> AAAAGAAGCCACCCTCCCGTCACCGACTTGAG;> TCATAAATCAGTTCAGAAAACGAGTCTAGCTGTGCCTGAGTACAAAAT;> ATTCATTGAATCCCCAAGAATAACTTAATTAAATAAGGAGAAACCA;> CATTACCGAGGGGGTAATAGTACACTATCA;> AAAATCAGAAATCACCTCAAATCACCATCAATGTCTGGAGTTTTT;> TTTTTTAAATTTAAAGAAGATGATGATTTTTTAACAAACATCAAG;> AGCCAGCATGAGGGAGGATAAAAATTTTTAGATAATCGTACAAACAAG;> TTCTGACCAATATATTTTAATGGAAACAGTTTTTTTACATAAATCAAT;> CCAGAGCCGCCATCTTGGCATTTTCGGTCTTTTTTTTTTATAGCCCCCTTATCCATCGAT;> TTAGTTAAAAGACAAACCGCGCCCAATAGCATCGTAGG;> TGATAGACGGTTTTTCGCCCTTTGACGTTGGAGTCCACGTTCTTTAATAGTGGACTCTTGTTCCAAACTGGAACAACACTCAACCCTATCTCGGGCTATTCTTTTGATTTATAAGGGATTTTGCCGATTTCGGAACCACCATCAAACAGGATTTTCGCCTGCTGGGGCAAACCAGCGTGGACCGCTTGCTGCAACTCTCTCAGGGCCAGGCGGTGAAGGGCAATCAGCTGTTGCCCGTCTCACTGGTGAAAAGAAAAACCACCCTGGCGCCCAATACGCAAACCGCCTCTCCCCGCGCGTTGGCCGATTCATTAATGCAGCTGGCACGACAGGTTTCCCGACTGGAAAGCGGGCAGTGAGCGCAACGCAATTAATGTGAGTTAGCTCACTCATTAGGCACCCCAGGCTTTACACTTTATGCTTCCGGCTCGTATGTTGTGTGGAATTGTGAGCGGATAACAATTTCACACAGGAAACAGCTATGACCATGATTACGAATTCGAGCTCGGTACCCGGGGATCCTCAACTGTGAGGAGGCTCACGGACGCGAAGAACAGGCACGCGTGCTGGCAGAAACCCCCGGTATGACCGTGAAAACGGCCCGCCGCATTCTGGCCGCAGCACCACAGAGTGCACAGGCGCGCAGTGACACTGCGCTGGATCGTCTGATGCAGGGGGCACCGGCACCGCTGGCTGCAGGTAACCCGGCATCTGATGCCGTTAACGATTTGCTGAACACACCAGTGTAAGGGATGTTTATGACGAGCAAAGAAACCTTTACCCATTACCAGCCGCAGGGCAACAGTGACCCGGCTCATACCGCAACCGCGCCCGGCGGATTGAGTGCGAAAGCGCCTGCAATGACCCCGCTGATGCTGGACACCTCCAGCCGTAAGCTGGTTGCGTGGGATGGCACCACCGACGGTGCTGCCGTTGGCATTCTTGCGGTTGCTGCTGACCAGACCAGCACCACGCTGACGTTCTACAAGTCCGGCACGTTCCGTTATGAGGATGTGCTCTGGCCGGAGGCTGCCAGCGACGAGACGAAAAAACGGACCGCGTTTGCCGGAACGGCAATCAGCATCGTTTAACTTTACCCTTCATCACTAAAGGCCGCCTGTGCGGCTTTTTTTACGGGATTTTTTTATGTCGATGTACACAACCGCCCAACTGCTGGCGGCAAATGAGCAGAAATTTAAGTTTGATCCGCTGTTTCTGCGTCTCTTTTTCCGTGAGAGCTATCCCTTCACCACGGAGAAAGTCTATCTCTCACAAATTCCGGGACTGGTAAACATGGCGCTGTACGTTTCGCCGATTGTTTCCGGTGAGGTTATCCGTTCCCGTGGCGGCTCCACCTCTGAAAGCTTGGCACTGGCCGTCGTTTTACAACGTCGTGACTGGGAAAACCCTGGCGTTACCCAACTTAATCGCCTTGCAGCACATCCCCCTTTCGCCAGCTGGCGTAATAGCGAAGAGGCCCGCACCGATCGCCCTTCCCAACAGTTGCGCAGCCTGAATGGCGAATGGCGCTTTGCCTGGTTTCCGGCACCAGAAGCGGTGCCGGAAAGCTGGCTGGAGTGCGATCTTCCTGAGGCCGATACTGTCGTCGTCCCCTCAAACTGGCAGATGCACGGTTACGATGCGCCCATCTACACCAACGTGACCTATCCCATTACGGTCAATCCGCCGTTTGTTCCCACGGAGAATCCGACGGGTTGTTACTCGCTCACATTTAATGTTGATGAAAGCTGGCTACAGGAAGGCCAGACGCGAATTATTTTTGATGGCGTTCCTATTGGTTAAAAAATGAGCTGATTTAACAAAAATTTAATGCGAATTTTAACAAAATATTAACGTTTACAATTTAAATATTTGCTTATACAATCTTCCTGTTTTTGGGGCTTTTCTGATTATCAACCGGGGTACATATGATTGACATGCTAGTTTTACGATTACCGTTCATCGATTCTCTTGTTTGCTCCAGACTCTCAGGCAATGACCTGATAGCCTTTGTAGATCTCTCAAAAATAGCTACCCTCTCCGGCATTAATTTATCAGCTAGAACGGTTGAATATCATATTGATGGTGATTTGACTGTCTCCGGCCTTTCTCACCCTTTTGAATCTTTACCTACACATTACTCAGGCATTGCATTTAAAATATATGAGGGTTCTAAAAATTTTTATCCTTGCGTTGAAATAAAGGCTTCTCCCGCAAAAGTATTACAGGGTCATAATGTTTTTGGTACAACCGATTTAGCTTTATGCTCTGAGGCTTTATTGCTTAATTTTGCTAATTCTTTGCCTTGCCTGTATGATTTATTGGATGTTAATGCTACTACTATTAGTAGAATTGATGCCACCTTTTCAGCTCGCGCCCCAAATGAAAATATAGCTAAACAGGTTATTGACCATTTGCGAAATGTATCTAATGGTCAAACTAAATCTACTCGTTCGCAGAATTGGGAATCAACTGTTATATGGAATGAAACTTCCAGACACCGTACTTTAGTTGCATATTTAAAACATGTTGAGCTACAGCATTATATTCAGCAATTAAGCTCTAAGCCATCCGCAAAAATGACCTCTTATCAAAAGGAGCAATTAAAGGTACTCTCTAATCCTGACCTGTTGGAGTTTGCTTCCGGTCTGGTTCGCTTTGAAGCTCGAATTAAAACGCGATATTTGAAGTCTTTCGGGCTTCCTCTTAATCTTTTTGATGCAATCCGCTTTGCTTCTGACTATAATAGTCAGGGTAAAGACCTGATTTTTGATTTATGGTCATTCTCGTTTTCTGAACTGTTTAAAGCATTTGAGGGGGATTCAATGAATATTTATGACGATTCCGCAGTATTGGACGCTATCCAGTCTAAACATTTTACTATTACCCCCTCTGGCAAAACTTCTTTTGCAAAAGCCTCTCGCTATTTTGGTTTTTATCGTCGTCTGGTAAACGAGGGTTATGATAGTGTTGCTCTTACTATGCCTCGTAATTCCTTTTGGCGTTATGTATCTGCATTAGTTGAATGTGGTATTCCTAAATCTCAACTGATGAATCTTTCTACCTGTAATAATGTTGTTCCGTTAGTTCGTTTTATTAACGTAGATTTTTCTTCCCAACGTCCTGACTGGTATAATGAGCCAGTTCTTAAAATCGCATAAGGTAATTCACAATGATTAAAGTTGAAATTAAACCATCTCAAGCCCAATTTACTACTCGTTCTGGTGTTTCTCGTCAGGGCAAGCCTTATTCACTGAATGAGCAGCTTTGTTACGTTGATTTGGGTAATGAATATCCGGTTCTTGTCAAGATTACTCTTGATGAAGGTCAGCCAGCCTATGCGCCTGGTCTGTACACCGTTCATCTGTCCTCTTTCAAAGTTGGTCAGTTCGGTTCCCTTATGATTGACCGTCTGCGCCTCGTTCCGGCTAAGTAACATGGAGCAGGTCGCGGATTTCGACACAATTTATCAGGCGATGATACAAATCTCCGTTGTACTTTGTTTCGCGCTTGGTATAATCGCTGGGGGTCAAAGATGAGTGTTTTAGTGTATTCTTTTGCCTCTTTCGTTTTAGGTTGGTGCCTTCGTAGTGGCATTACGTATTTTACCCGTTTAATGGAAACTTCCTCATGAAAAAGTCTTTAGTCCTCAAAGCCTCTGTAGCCGTTGCTACCCTCGTTCCGATGCTGTCTTTCGCTGCTGAGGGTGACGATCCCGCAAAAGCGGCCTTTAACTCCCTGCAAGCCTCAGCGACCGAATATATCGGTTATGCGTGGGCGATGGTTGTTGTCATTGTCGGCGCAACTATCGGTATCAAGCTGTTTAAGAAATTCACCTCGAAAGCAAGCTGATAAACCGATACAATTAAAGGCTCCTTTTGGAGCCTTTTTTTTGGAGATTTTCAACGTGAAAAAATTATTATTCGCAATTCCTTTAGTTGTTCCTTTCTATTCTCACTCCGCTGAAACTGTTGAAAGTTGTTTAGCAAAATCCCATACAGAAAATTCATTTACTAACGTCTGGAAAGACGACAAAACTTTAGATCGTTACGCTAACTATGAGGGCTGTCTGTGGAATGCTACAGGCGTTGTAGTTTGTACTGGTGACGAAACTCAGTGTTACGGTACATGGGTTCCTATTGGGCTTGCTATCCCTGAAAATGAGGGTGGTGGCTCTGAGGGTGGCGGTTCTGAGGGTGGCGGTTCTGAGGGTGGCGGTACTAAACCTCCTGAGTACGGTGATACACCTATTCCGGGCTATACTTATATCAACCCTCTCGACGGCACTTATCCGCCTGGTACTGAGCAAAACCCCGCTAATCCTAATCCTTCTCTTGAGGAGTCTCAGCCTCTTAATACTTTCATGTTTCAGAATAATAGGTTCCGAAATAGGCAGGGGGCATTAACTGTTTATACGGGCACTGTTACTCAAGGCACTGACCCCGTTAAAACTTATTACCAGTACACTCCTGTATCATCAAAAGCCATGTATGACGCTTACTGGAACGGTAAATTCAGAGACTGCGCTTTCCATTCTGGCTTTAATGAGGATTTATTTGTTTGTGAATATCAAGGCCAATCGTCTGACCTGCCTCAACCTCCTGTCAATGCTGGCGGCGGCTCTGGTGGTGGTTCTGGTGGCGGCTCTGAGGGTGGTGGCTCTGAGGGTGGCGGTTCTGAGGGTGGCGGCTCTGAGGGAGGCGGTTCCGGTGGTGGCTCTGGTTCCGGTGATTTTGATTATGAAAAGATGGCAAACGCTAATAAGGGGGCTATGACCGAAAATGCCGATGAAAACGCGCTACAGTCTGACGCTAAAGGCAAACTTGATTCTGTCGCTACTGATTACGGTGCTGCTATCGATGGTTTCATTGGTGACGTTTCCGGCCTTGCTAATGGTAATGGTGCTACTGGTGATTTTGCTGGCTCTAATTCCCAAATGGCTCAAGTCGGTGACGGTGATAATTCACCTTTAATGAATAATTTCCGTCAATATTTACCTTCCCTCCCTCAATCGGTTGAATGTCGCCCTTTTGTCTTTGGCGCTGGTAAACCATATGAATTTTCTATTGATTGTGACAAAATAAACTTATTCCGTGGTGTCTTTGCGTTTCTTTTATATGTTGCCACCTTTATGTATGTATTTTCTACGTTTGCTAACATACTGCGTAATAAGGAGTCTTAATCATGCCAGTTCTTTTGGGTATTCCGTTATTATTGCGTTTCCTCGGTTTCCTTCTGGTAACTTTGTTCGGCTATCTGCTTACTTTTCTTAAAAAGGGCTTCGGTAAGATAGCTATTGCTATTTCATTGTTTCTTGCTCTTATTATTGGGCTTAACTCAATTCTTGTGGGTTATCTCTCTGATATTAGCGCTCAATTACCCTCTGACTTTGTTCAGGGTGTTCAGTTAATTCTCCCGTCTAATGCGCTTCCCTGTTTTTATGTTATTCTCTCTGTAAAGGCTGCTATTTTCATTTTTGACGTTAAACAAAAAATCGTTTCTTATTTGGATTGGGATAAATAATATGGCTGTTTATTTTGTAACTGGCAAATTAGGCTCTGGAAAGACGCTCGTTAGCGTTGGTAAGATTCAGGATAAAATTGTAGCTGGGTGCAAAATAGCAACTAATCTTGATTTAAGGCTTCAAAACCTCCCGCAAGTCGGGAGGTTCGCTAAAACGCCTCGCGTTCTTAGAATACCGGATAAGCCTTCTATATCTGATTTGCTTGCTATTGGGCGCGGTAATGATTCCTACGATGAAAATAAAAACGGCTTGCTTGTTCTCGATGAGTGCGGTACTTGGTTTAATACCCGTTCTTGGAATGATAAGGAAAGACAGCCGATTATTGATTGGTTTCTACATGCTCGTAAATTAGGATGGGATATTATTTTTCTTGTTCAGGACTTATCTATTGTTGATAAACAGGCGCGTTCTGCATTAGCTGAACATGTTGTTTATTGTCGTCGTCTGGACAGAATTACTTTACCTTTTGTCGGTACTTTATATTCTCTTATTACTGGCTCGAAAATGCCTCTGCCTAAATTACATGTTGGCGTTGTTAAATATGGCGATTCTCAATTAAGCCCTACTGTTGAGCGTTGGCTTTATACTGGTAAGAATTTGTATAACGCATATGATACTAAACAGGCTTTTTCTAGTAATTATGATTCCGGTGTTTATTCTTATTTAACGCCTTATTTATCACACGGTCGGTATTTCAAACCATTAAATTTAGGTCAGAAGATGAAATTAACTAAAATATATTTGAAAAAGTTTTCTCGCGTTCTTTGTCTTGCGATTGGATTTGCATCAGCATTTACATATAGTTATATAACCCAACCTAAGCCGGAGGTTAAAAAGGTAGTCTCTCAGACCTATGATTTTGATAAATTCACTATTGACTCTTCTCAGCGTCTTAATCTAAGCTATCGCTATGTTTTCAAGGATTCTAAGGGAAAATTAATTAATAGCGACGATTTACAGAAGCAAGGTTATTCACTCACATATATTGATTTATGTACTGTTTCCATTAAAAAAGGTAATTCAAATGAAATTGTTAAATGTAATTAATTTTGTTTTCTTGATGTTTGTTTCATCATCTTCTTTTGCTCAGGTAATTGAAATGAATAATTCGCCTCTGCGCGATTTTGTAACTTGGTATTCAAAGCAATCAGGCGAATCCGTTATTGTTTCTCCCGATGTAAAAGGTACTGTTACTGTATATTCATCTGACGTTAAACCTGAAAATCTACGCAATTTCTTTATTTCTGTTTTACGTGCAAATAATTTTGATATGGTAGGTTCTAACCCTTCCATTATTCAGAAGTATAATCCAAACAATCAGGATTATATTGATGAATTGCCATCATCTGATAATCAGGAATATGATGATAATTCCGCTCCTTCTGGTGGTTTCTTTGTTCCGCAAAATGATAATGTTACTCAAACTTTTAAAATTAATAACGTTCGGGCAAAGGATTTAATACGAGTTGTCGAATTGTTTGTAAAGTCTAATACTTCTAAATCCTCAAATGTATTATCTATTGACGGCTCTAATCTATTAGTTGTTAGTGCTCCTAAAGATATTTTAGATAACCTTCCTCAATTCCTTTCAACTGTTGATTTGCCAACTGACCAGATATTGATTGAGGGTTTGATATTTGAGGTTCAGCAAGGTGATGCTTTAGATTTTTCATTTGCTGCTGGCTCTCAGCGTGGCACTGTTGCAGGCGGTGTTAATACTGACCGCCTCACCTCTGTTTTATCTTCTGCTGGTGGTTCGTTCGGTATTTTTAATGGCGATGTTTTAGGGCTATCAGTTCGCGCATTAAAGACTAATAGCCATTCAAAAATATTGTCTGTGCCACGTATTCTTACGCTTTCAGGTCAGAAGGGTTCTATCTCTGTTGGCCAGAATGTCCCTTTTATTACTGGTCGTGTGACTGGTGAATCTGCCAATGTAAATAATCCATTTCAGACGATTGAGCGTCAAAATGTAGGTATTTCCATGAGCGTTTTTCCTGTTGCAATGGCTGGCGGTAATATTGTTCTGGATATTACCAGCAAGGCCGATAGTTTGAGTTCTTCTACTCAGGCAAGTGATGTTATTACTAATCAAAGAAGTATTGCTACAACGGTTAATTTGCGTGATGGACAGACTCTTTTACTCGGTGGCCTCACTGATTATAAAAACACTTCTCAGGATTCTGGCGTACCGTTCCTGTCTAAAATCCCTTTAATCGGCCTCCTGTTTAGCTCCCGCTCTGATTCTAACGAGGAAAGCACGTTATACGTGCTCGTCAAAGCAACCATAGTACGCGCCCTGTAGCGGCGCATTAAGCGCGGCGGGTGTGGTGGTTACGCGCAGCGTGACCGCTACACTTGCCAGCGCCCTAGCGCCCGCTCCTTTCGCTTTCTTCCCTTCCTTTCTCGCCACGTTCGCCGGCTTTCCCCGTCAAGCTCTAAATCGGGGGCTCCCTTTAGGGTTCCGATTTAGTGCTTTACGGCACCTCGACCCCAAAAAACTTGATTTGGGTGATGGTTCACGTAGTGGGCCATCGCCC;> AACGGAGATTTGTATTAGGAATACAAAAGGATCAGGACGATGCCACT;> TTTTTGCGCGAAACACTAAAACCAGCGATAAGAGGCAGAGGACTAAAGACTTT;> TTGAGATTTTGTGAATTATACCAGAACGTAACCAGCATCGGAACGAGG;> CTGACCTTCATCGCCTCCATGTTAATTACGAGCGTTTACCAGACGACG;> GTAATCTTGACAAGATTGAAAGACTCCAAAACTAAAGGATTTTCACGGCTGAGGC;> TTTTGTTTTGTCCAGACAGCCCTCATTTTTTTTTTTAGTTAGCGTAAC;> AGACGTTAGTAAATGAATTGTATTCTTAAAC;> CGGTTTATCAGCTTGTTGAAAATTTTTT;> GTTTCAGCAGCTTGATCATCGCCCACGCATAAGCATGATTAACAGTTA;> GGAGTGAGTTGCGGGATCGTCACCCCCGTATA;> GTGAATAAGGCTTTTTTTTTTTTGCCCTGACGAGAAAACCCATGTCAGGGAT;> TCATTCATGGTTTAATTTCAACTTTAATCAAATTTTCT;> AAAGCTGCTTCAACAGTATGGGATTTTGCTGATCTAAAGCTTGAGA;> ACCGGATAGGAACAAAAAAGGCTCCAAAAGGAGCCTTTCATCAAGA;> GGTCAATCGACCAACTGAGGCTTTTTGCAGGGTTCGGAACCTATTATT;> TACGTTAATAAAATTTTTTTTTTCGAACTAACGGAACCTCATTTTTTT;> TTGGGAAGGGCTCATTACCTTATGCGATTTACACCAGATTACAGGT;> CAAAATAGCAGATACATAACGCCCACATTCAACTAATCAACATTATTTTT;> AAAAGCCTACCAGTATAAAGCCATATCATTCTGCAGAACGCTGAGAC;> TTACTAGACGGAATCGCCAACATGCAGAAGCAAAGCGGAT;> TTTTTCGTTAAATATGGTTTGAAATATTTTTTCCGACCGTGTGAT;> ACGAAGGCGTACCGACTTTTGCCAATTAGCAAGGCCGGAACCGTAATC;> AAAACGAAATCCGCGCGCAGACAGGCGCATAGGCTGG;> AAATTCTTGTTTAGTATCATATGAAAGAATAAAATGTTTAGCCAGTA;> CCATTAAATAGTACCGGTGCCGTCTTACCAGCGCCAAAGA;> TTCATGAGAACGAGGACCTGCTGATAAATTGTGTCGATATACCAATACAGACC;> GGTATTAAACCAAGTCGTTATACCATTTTCGAGACTGGA;> TCGGCTGTCTTTCCTACGCTCAATAACAACG;> CAGTACAACAATAGGTAAGAACTAAAAATCAGAAAGATTCATCAG;> CGCCTGTATTCGTCACAGTATAGCCCGGATTTTTTTTTTATAGGTGTATCAC;> GCCGCTTAATAGAAATTCATTACCCAAATCCTTAGCCGGGAAGTTT;> AGTTAAAGTTCGGTCCTTTCGAGGTGAATT;> CCAGCTACAGCGTCTTTCCAGAGTAGACGGGGAACAAAG;> TTTTGCATTCCAGGTAATAAGTTTTTTTTTTTTTTAACGGGGTCAGTG;> AAGACTCCAATACATACATAAAGGTGGAAAGCATAAATCC;> GAGGAAACGCTAACGAATTTTATCCTGAATACCGCACT;> TATCCCAACAGATATAGAGTACCTTTAATTGCTGTACCAACATTAACAGAACCTAC;> TATTATTGCCAGTTACAAGATTAGTTGCTATTATTTTC;> AACAGTGCTCAGCAGCAACAACACCGATAGTTGCGCCGTCTTTCC;> GAAGGCTTATCCGGTCCTTAAATCAAAATAGAACCTCCGAGAGAAT;> ATTCTAAGAACGCTTTTTTGAGGCGTTTTAGCATATAACTTAACCTCC;> GCGGATAAAAAAGGTAACGGAAATTATTCATT;> TTAGGATTCAATAAACGTTTTAATGTCTTTACGATTCAAAAGGGTGAG;> AAGCAAATGCGCCTGTAAGAGGAAGCCCGAAAAAATGCAAAAACATTA;> CAGCTAACAAGAACGACAAGCAAGCCGTTTTTTTGCACATTAAGAGTTACCAGA;> TTATCAACAATAGATATCAATAAAATCATTCCATCCTATTTTGAAG;> AAGTCCTGAACAATTTTTTGAAAAATAATATCAGAACGCGATGCAAAT;> AGAACCGCCACCCTTTTTTTTTTTCAGAGCCACCACTAGCGTTTTTTT;> ATATAAAACCAACCTTAACCCTGCATAGTAAGAGCAACAAAGTAC;> ATAAGAGACTGTCCAGACGACGAAGCGGGGT;> CCATATTCAGTAGGGACACCGGAATCATAA;> CAGGAAGAACAATAATTTGAATTACCTTTT;> ATGAATATTAGATTTTGTTATTAATTTTATTTTTTTTTTAAAGTTTGAGTAA;> GTAAACGTAGGGTTATCCAATAAATCATAC;> CCAATAGGTGTTAAATTCGGCCTCACCGCTTCCAGCAACCGCAAGAATTGGGTAAA;> ACTTCTGACATCTGCCCCGTCGGAAAGGGAAGAAAGCGAAAGCGGTCA;> TGGATTATCATATCAAAATTATTTTTGTATA;> GATTGTTGAGTCAATAGTGAATGGCTTAGGGACCATTGTTAAGCC;> TTTTTAACGCCATAACGGCGGATTGACCGCGGGGAAA;> AACTGTTGGGAAGTTTTTTTTTTGGCGATCGGTGCGTCGTCTCGTCCGGCAA;> GGCCTCTTCGCTATTCTTTGAATGATAATCTGACCCTG;> CAACCGATAAGACACCATAAAGCCTCAGAGCATTGTTAAACATATGTA;> CGGAAGCAAACTCCAACAGGTCAGAAAGATT;> GATACAGGGGAGGTTGCCTCAGAGCCGCCTTTTTTTTTTACCAGAACCACCAACCGGAAC;> GAAAATTCCGTAGAATTATTACGCAGTATGGACAATGAACTACAAAAACAACT;> TTTGTCACAATCAATAACAAACAAGCAGTCTC;> ACGGAATATATAAAATACCCAAAAGAACTGCCGATATA;> GTCATTTTTCGAGCTTTTTGCGGGAGAAGCCTTTATTTCATTAAGCA;> TTTTTAGTGTACTAGTAAGCGTCATATTTTTTTTTTCATGGCTTTTGATTTGGCCTT;> TGGCAACAAGTTTATATGCCCCCGTACCAGGTAGCAACGGCTACA;> GCTTAGAGCTTAATTAGGAAACCGATAGCCAGAATTAATGAGCGC;> GCTGAATACAACTAAAAGTAGTAGTAACCTGTTCTGGCCTTCCTGTAG;> TGAATTTACCGTTCCTTAGCAAACAGACGACCTTGAGTTGATATA;> ATTAAGACTCTGTAAAAGCAAATATTTAAATTGGCAAAGCAGTTTGAG;> ATAGCGATAGCTTAGTAGCTCAAGATTAGA;> TCATTAAAGCCGCCACAAAAGGGCGACATTTTTGCTCATGCCTAT;> TAAAGCTATAATACTCAAAGCGAACCAGACTCCTCAAGTGAAAGT;> AATCGGTTCCTTTTGATAAGAGCTGAAACAAGAAGGACATCGAGA;> TCGTCGCTATTAATTCCAATCGCTTGGGTTAACAGCCA;> AATTTTCCCTTAGTTTTTTAATCCTTGAAAACAAACAGAATCATCAAT;> CCACCACAGGCAGGTCAAAATCCGTACTCAGGAGGTTCGGGTAAACGAAAGA;> CCCTCAGAAACCGCCTCCCTCAGAAGTTTGCCCATTTGG;> ACCTTGCTCAATTTCACGGATTCGCCTGATTG;> ACCACCGGACCGCCACCCTCAGAGGATATTC;> ACCCTCATAGGTAAACCTGACTATAAATCATAGCGTCCAATACTG;> TTTCATCTTCATAATAATGAAAGCGAGAGGCTTTTGCATAAAAACATACGTA;> TCAGACTGTAGCGCGTCAGAGCCAAAGGTGAATATGGTGAGAGGGT;> CTTTAGCGAGTAGCGACAGAATCAGAGACAGAGTAGCACGAATTAG;> AAAGGCCGACGCAAGGGAAGGTAAATATTGAAGTAATT;> TAATGTGTATATTTTGACTTCAAATATCGCAACATGTTGCAGAGG;> ACATTTAAATAAATTATCTACAAAGGCTATCATAAAACGATGGCGAAA;> AGCAGCAACGTCACCATTATCAAGAACCGCCACCCTCAGCAAGCC;> ATGATATTCAACCGTAATGACCATTATAGTTAATTTAG;> ATGCCGGAGAGGGTACTCAAATGTTTCATCGAGAATCG;> CCCTGAACCTTACCAACGCAATAATAACGGAAGAAACGCA;> TTTTTAAAGTCAGATCTTACCGAAGCTTTTTTTTTTCCTTTTTAAGAAA;> TAATATCAGAGAGATAAAGAGCAATCCAAATATAAATATGTAATGCTG;> GAAATAGCAATAGCTAGGGTAATCTGAACA;> GAAACAATTCTGCGAACGAGTAGAATGGTCAAGCTGAGAA;> CAATAATACCCACAAAACAGGGAAGCGCATCCTAATTT;> AGAAACGATTTTTTGAACATAAAGAATTGACCTTT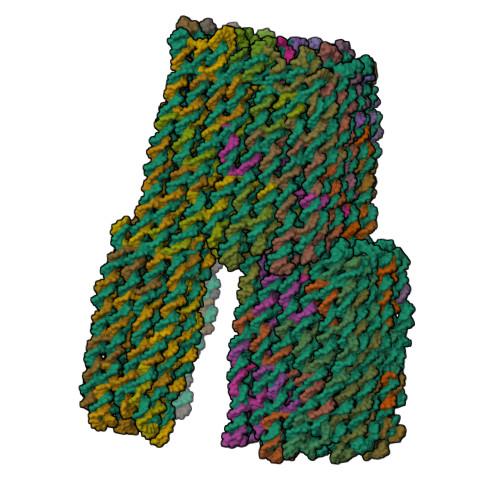ACATTTTT;> TTTAACGTCAAAATTTTTTATGAAAATAGCAGTACCTTTTTTTTT;> GTTTCATTTGCGGATGAGGCAAGGCAAAGAATTAGCAAAAGCCAGAA;> TTTTCCATATAATTTGGGGCGCGAGTTTTTTTTTTCTGAAAAGGTGGC;> TTAGCTATATTTTCACAGTTGATTCTGGAAAGTAAGCA;> AGATACATTTCGCAATTTAGTTTCATGTTT;> TTATCAAAATCATTTTTTTAGGTCTGAGAGACATGGCAATTTTTT;> TTTTTCTGAGCAAGAATTGAGGAAGGTTTTTTTTTTTTATCTAAAATAT;> CGCGCAGACAACTAATCGGCCAGTGAACGGATAACCTCAC;> ATTCATTAAAACAAAATTAATTTGCATCAACTTTAAA;> TCAATTACTTTTACATTACATTTGAGGATTTTTTTTTTTTTAGAAGTATTAG;> CGGGAGAAACGTCAGATATGTGAGTGAATA;> AGAAAAGCCCCAAAAACGACAACTAGATTAGATTTTGAAT;> CCTTCTGACTTGCTGGATTAGTAATAACATTTTTTTTTTTCACTTGCCTGAGTTTTTATA;> ACTTTCTCCGGCCTTTAGTGATGAAGGGTAAACTTAAATGAGACGCA;> AATTTGTGAGAGATAGCGGAAAAATTCTGCTC;> ATCGGCGCCAGTCACGACGTTGGGTCATTGACCAAGT;> TTTTTGTTGAAAGCTCAATCAATATCTTTTTTTTTTTGGTCAGTTGGCATACCGAAC;> TTTTTAAAAAAGCTTGGGCGGATAAAAAAAAGGGATAGCTCTCA;> ACTGATAGGGCTATTAATTCACCAGGAAAAACGCTCATGGCCATCAC;> CCCTAAAACAGCAGAATGCTGAACCTCAAATATCAAACCGTGGAGCC;> CATCGCCAGCCACGGGCCAAGCTTTCAGAGGCTATTTT;> TTAAAAACTTTAGGAGCACTAAGGCGAATTTGAGAGA;> ACGCCAGCGCCATTCGCACATCCTCATAACGG;> AGGCGATTGGGTTTTCAAACGTACAGCGCCAT;> GGGGGATGTGCTGCAAGAATCGACCTGAGA;> CAACAGCTCGTGCCAGCTGCTTTTTTTTTTATTAATGAATCGGCCAGTCGGTTCACGGT;> GGGAACACAAAAATATTTTTAAATCAATTCTACTAATGTACGGTGTCCCAAT;> GTAACAACAAACCACCTAAACAGGAGGCCGATGCCGCGCT;> GGGCGCCAGGATCCCCGGGTACCGCCTCCTC;> TAGATGGGGCCTGGGGTGCCTAATAAGCACTAGAGCTTGAGGGTCGAGTTTTT;> CGCATCGTAACCGTGATAATGGAATTCGCG;> ATCATCATATTCCTTTTTTTTTTTGATTATCAGATGGTGCTTTCTTTTT;> TCATGGTCATACCGGGGGTTTTTTTTTTTTTCTGCCAGCACGCGGGCCGTTTTTTT;> ATTCGTAACGGGGAGAGGCGGTTTCACCAGT;> AGGAAGATCAACATACGAGCCGGATCCCTTAC;> GAACAAAGCGTATTAATAGAACGTCAGCGTGGGCAAATTA;> ATCCTTTGCCCGAACCAGGTTTAGCACGTA;> CAGCTTAGTGCCTGTTCTTCGCGTCCGTGAGAGCTCGATGTGAAATGCGTTGCG;> GTCGGTGGTGCCATCCAGCATCAGCAGATGCCCCCTGCATTAAATCAA;> TGCTGGTCTTTTAGAGGGACGACGACAGTACAGCTCATTAATATT;> TGTTATCCAACGGCATCGGGGTCAGCGCGGTTCAGACGATCCAGCGCA;> GCTCACAACAGCACCACAGTTGAAGCCAGCTTTCCGGC;> AGCATAAATGGTCAGTGGTGCCGGAAACCA;> CAGGAACGGTACGCCAAGGCCACCACCGTTGT;> TAGAAGAACTCGTTAGACTATGGTCGTATAACGGCGCTGGCAAGTGT;> TTTTGAAACCTGTCCAGTTTGGAACTTTTTTTTTTAAGAGTCCACTAT;> GCCTGGCCCTGAGAGACCAGCAGGAAAGGGCGACGTGAACGCGGTATG;> AAGCGGTTAATGGGAGGGTGGTTTTTCTTTTGCGTATTCATTAATT;> GCCGGCGACCGATTTAAATCGGAACCCTAAAGATAAACA;> AGGAGCGGCGGGAGCAGAAGGAGCGGAATTATAATCCTCATCAAC;> TGGTGGTTGATTGCCCTTCACCGAGACGGG;> CGCTGCGCGTAACCACGGAGCCCACGTGGCGGTGTAAA;> GTGGACTCTCACTGCCCGCTTTCCAACGCG;> CCAACGTCCGAAAATCATCCCTTACATCACCCAAATCAAG;> TAATGCGCCGCTACAGATCAGTGGAATCCTGGGACTTG;> GGCGCGTAATCAGAGGCGCTAGATTAAATGTGAGCGACCAGCTTT;> CTGTGGTGCTGCGTTTTTTTTTTGCCAGAATGCGGCTGCGCGCCTTTT;> ACTGGTGTGCCCTGCGGTGCCGTAGGGCGATGGCCCACTAAAAACCGAATCGTT;> GAGTAAAAGAGTCTGTCACACCCTAAAGGGAAGAAAGGTTCTCCGT;> GCTTTCGGCCAACGGTTCCACACGCACTCCTAGGTCACGTTGGTG;> GGTTTCTTTGCTCGTCAAATACCAGCCTCCGCGTTTTT;> AGCAATACCCAGCCAAACGTGCCACAATATGCCGTCAATAGATAA;> TTCTTTGTAATATCCAGAAGTGCATTATCATTTTGCG;> GTGTCACCGGCTGGAGGTGTCCCACGCAACTTTCCTG;> TTTTTGCTGGTAACACTCAATCCGCCGGTTGCAGGC;> AGCCGGGTCACTGTTGTTCAGCATCTATCAGAGTGAGC;> TAGGGTTGTGTGCACTAGCGGTGCCGGTGCCGGGTTACC;> AAGAATAGCCCGAGATAAAGAACTGCAGCCCATAGCTG;> TTTTTAGTGTTGTTCCGAAATCGGCAAACTGTTTGA;> TTTTTTGCCACGCTGGTTTGCCGTTGCAGCTAACTCA;> TTGCAACAGTCACACGACCAGTAAGAACCAC;> TAAAAGGTGGCACAGAGAACAAACTTTACAAACAATT;> GTCTTTAAGCCAGAGCCATTCAGGCTGCGCCCCCGGTTTGAACGG;> TTTTTTCGCTGGCTACATTTTAAATGGATTATTTACAGGCGGTCACGCGGTC;> AATCAACAAGAATACGGACATTCTGGCCATTTTTTTTTTACAGAGATAGAACTATTACCG;> ATTTGCCGCCAGCAGCGCACAGGCGTGGTGATCCCGTATTTTT;> AGTATTAAAGCAGCAAATGAAAAATCTAAAGCGGAAACATGCGCGA;> GAAACAGCGCCACGCGTTTACCAGATGCTGATTGCCGT;> TGAGAGCCCACCGCCTGCAACAGTGGATCAAAGTTAAACGTCCCGG;> CATCACCTGATAAAACAGAGGTGATTGGCAG>[2x]LSEEEIQRIFGLSSEQIKSLPEEXY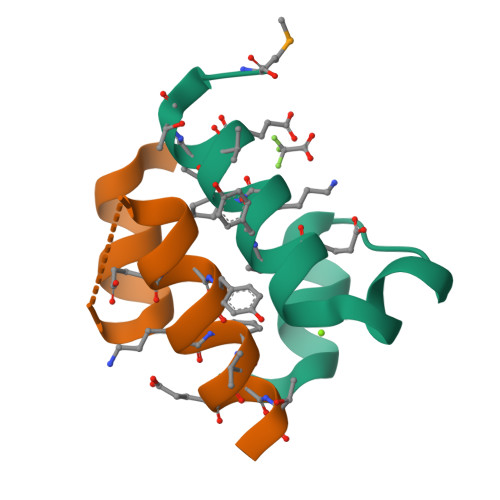KKXVEXTGYM N-[(3R)-3-amino-4-(2,4,5-trifluorophenyl)butyl]-3'-(trifluoromethyl)biphenyl-4-carboxamide | C24 H20 F6 N2 O | 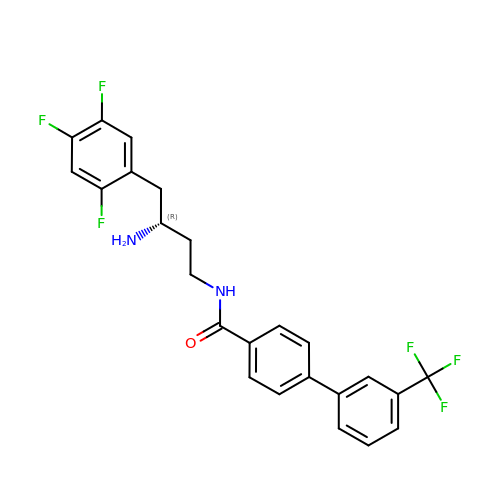UPWUIPKOGKXOGK-IBGZPJMESA-N The cysteine desulfurase IscS is a highly conserved master enzyme initiating sulfur transfer via persulfide to a range of acceptor proteins involved in Fe-S cluster assembly, tRNA modifications, and sulfur-containing cofactor biosynthesis. IscS is a highly conserved, widely distributed pyridoxal-5′-phosphate (PLP)-dependent enzyme, with 60% sequence identity between the enzyme from Escherichia coli and its human homolog, NFS1. It initiates intracellular sulfur trafficking, delivering the sulfur to several sulfur-accepting proteins such as IscU, ThiI, TusA, and MoaD/MoeB that commit the sulfur to different metabolic pathways, including iron-sulfur cluster assembly, thiamine and biotin synthesis, tRNA modifications, or molybdopterin biosynthesis. The small domain (residues 1–15 and 264–404) contains the critical active site cysteine Cys328.

We have determined the structure of PLP-bound IscS at 2.05 Å resolution in a different crystal environment from that observed previously and have also found the Cys328IscS-containing loop extending away from the protein with its tip disordered. Therefore, IscS prefers an “open” conformation of the Cys328 loop, compatible with sulfur transfer to an acceptor. In contrast, the analogous loops in two other cysteine desulfurases, NifS and SufS, are shorter and prefer a closed conformation, with the active site cysteine residue located in proximity to PLP, compatible with loading of sulfur acquired from bound cysteine substrate. We postulate that the longer Cys328 loop found in IscS is essential for this enzyme to transfer sulfur to multiple acceptors. Easily recognizable electron density in our structures indicated the presence of the PLP cofactor as an internal aldimine covalently bound to Lys206, as previously observed. IscS is composed of two domains. Dimerization of IscS predominantly involves residues from the large domain.

>MGSSHHHHHHGSMYGVYRAMKLPIYLDYSATTPVDPRVAEKMMQFMTMDGTFGNPASRSHRFGWQAEEAVDIARNQIADLVGADPREIVFTSGATESDNLAIKGAANFYQKKGKHIITSKTEHKAVLDTCRQLEREGFEVTYLAPQRNGIIDLKELEAAMRDDTILVSIMHVNNEIGVVQDIAAIGEMCRARGIIYHVDATQSVGKLPIDLSQLKVDLMSFSGHKIYGPKGIGALYVRRKPRVRIEAQMHGGGHERGMRSGTLPVHQIVGMGEAYRIAKEEMATEMERLRGLRNRLWNGIKDIEEVYLNGDLEHGAPNILNVSFNYVEGESLIMALKDLAVSSGSACTSASLEPSYVLRALGLNDELAHSSIRFSLGRFTTEEEIDYTIELVRKSIGRLRDLSPLWEMYKQGVDLNSIEWAHH[2x]> MTGYLTIGGQRYQAEINDLENLGEMGSGTCGQVWKMRFRKTGHVIAVKQMRRSGNKEENKRILMDLDVVLKSHDCPYIVQCFGTFITNTDVFIAMELMGTSAEKLKKRMQGPIPERILGKMTVAIVKALYYLKEKHGVIHRDVKPSNILLDERGQIKLCDFGISGRLVDSKAKTRSAGCAAYMAPERIDPPDPTKPDYDIRADVWSLGISLVELATGQFP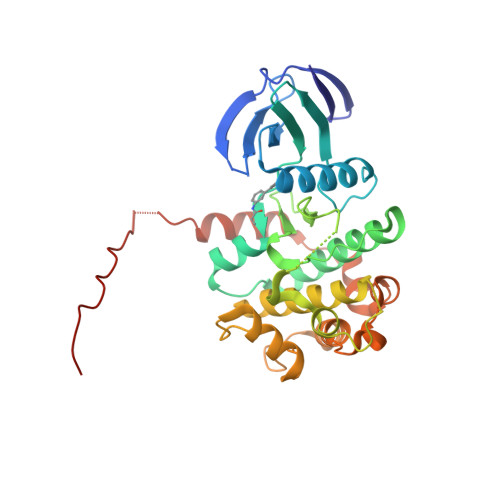YKNCKTDFEVLTKVLQEEPPLLPGHMGFSGDFQSFVKDCLTKDHRKRPKYNKLLEHSFIKRYETLEVDVASWFKDVMAKTESPRTSGVLSQPHLPFFRHHHHHH> ICI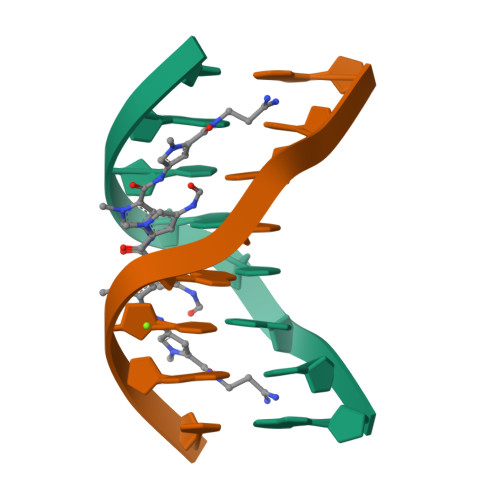TACIC>MAVNSKYHHSCINCGGLNTDERNERGLPCEVCLPEDSPSDIYRALLERKTLKEYRFYHEFWNEYEDFRSFFKKKFGKDLTGYQRLWAKRIVQGKSFTMVAPTGVGKTTFGMMTALWLARKGKKSALVFPTVTLVKQTLERLQKLADEKVKIFGFYSSMKKEEKEKFEKSFEEDDYHILVFSTQFVSKNREKLSQKRFDFVFVDDVDAVLKASRNIDTLLMMVGIPEEIIRKAFSTIKQGKIYERPKNLKPGILVVSSATAKPRGIRPLLFRDLLNFTVGRLVSVARNITHVRISSRSKEKLVELLEIFRDGILIFAQTEEEGKELYEYLKRFKFNVGETWSEFEKNFEDFKVGKINILIGVQAYYGKLTRGVDLPERIKYVIFWGTPSMRFSLELDKAPRFVLARVLKEMGLIKAQENPDVEELRKIAKEHLTQKEFVEKVKEMFRGVVVKDEDLELIIPDVYTYIQASGRSSRILNGVLVKGVSVIFEEDEEIFESLKTRLLLIAEEEIIEEAEANWKELVHEVEESRRRSERELTDTSRSLLIIVESPTKAETLSRFLGRASSRKERNIIVHEAVTGEGVILFTATRGHVYDLVTKGGIHGVEEENGKFVPVYNSLKRCRDCGYQFTEDRDECPVCSSKNIDDKTETLRALREISLEADEILVATDPDVEGEKISWDVTQYLLPSTRSLRRIEMHEITRYGFKKARESVRFVDFNLVKAQIVRRVQDRWIGFELSGKLQKRFGRSNLSAGRVQSTVLGWIVEREEEYKKSEKDFTLLVLENGVNLEVEGKIADDVVTVVELQEAEEEKNPLPPYTTSSALSEISQKLRLGVQEVMDILQDLFEKGFITYHRTDSTRISLEGQNVARTYLRKIGKEDIFMGRSWSTEGAHEAIRPVKPIDARELEEMIEEGLIADLTKKHLRVYELIFNRFLASQSAAVKVKKQIVTVDVDGKRMGIEQIVEILRDGWNLFVPLTVSPRFEHRTYKIKEKKFYKKHTVPLFTQASIVEEMKKRGIGRPSTYAKIVEVLFRRGYVYEDKYKRVRPTRFGVMVYSYLKERYEKYVTEETTRRLEEIMDKVERGEEDYQATLRLL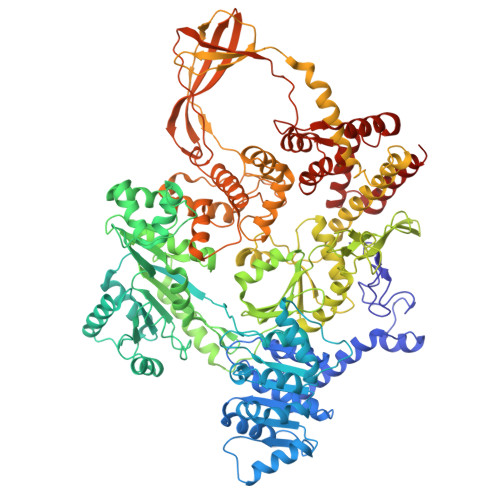YEEIKSLMEEG[2x]> MEKETGPEVDDSKVTYDTIQSKVLKAVIDQAFPRVKEYSLNGHTLPGQVQQFNQVFINNHRITPEVTYKKINETTAEYLMKLRDDAHLINAEMTVRLQVVDNQLHFDVTKIVNHNQVTPGQKIDDESKLLSSISFLGNALVSVSSDQTGAKFDGATMSNNTHVSGDDHIDVTNPMKDLAKGYMYGFVSTDKLAAGVWSNSQNSYGGGSNDWTRLTAYKETVGNANYVGIHSSEWQWEKAYKGIVFPEYTKELPSAKVVITEDANADKNVDWQDGAIAYRSIMNNPQGWEKVKDITAYRIAMNFGSQAQNPFLMTLDGIKKINLHTDGLGQGVLLKGYGSEGHDSGHLNYADIGKRIGGVEDFKTLIEKAKKYGAHLGIHVNASETYPESKYFNEKILRKNPDGSYSYGWNWLD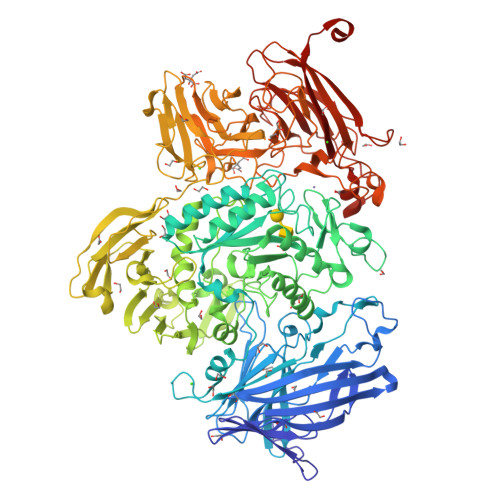QGINIDAAYDLAHGRLARWEDLKKKLGDGLDFIYVNVWGNGQSGDNGAWATHVLAKEINKQGWRFAIEWGHGGEYDSTFHHWAADLTYGGYTNKGINSAITRFIRNHQKDAWVGDYRSYGGAANYPLLGGYSMKDFEGWQGRSDYNGYVTNLFAHDVMTKYFQHFTVSKWENGTPVTMTDNGSTYKWTPEMRVELVDADNNKVVVTRKSNDVNSPQYRERTVTLNGRVIQDGSAYLTPWNWDANGKKLSTDKEKMYYFNTQAGATTWTLPSDWAKSKVYLYKLTDQGKTEEQELTVKDGKITLDLLANQPYVLYRSKQTNPEMSWSEGMHIYDQGFNSGTLKHWTISGDASKAEIVKSQGANDMLRIQGNKEKVSLTQKLTGLKPNTKYAVYVGVDNRSNAKASITVNTGEKEVTTYTNKSLALNYVKAYAHNTRRNNATVDDTSYFQNMYAFFTTGADVSNVTLTLSREAGDEATYFDEIRTFENNSSMYGDKHDTGKGTFKQDFENVAQGIFPFVVGGVEGVEDNRTHLSEKHDPYTQRGWNGKKVDDVIEGNWSLKTNGLVSRRNLVYQTIPQNFRFEAGKTYRVTFEYEAGSDNTYAFVVGKGEFQSGRRGTQASNLEMHELPNTWTDSKKAKKATFLVTGAETGDTWVGIYSTGNASNTRGDSGGNANFRGYNDFMMDNLQIEEITLTGKMLTHHHHHH> ACTKNAIAQTGFNKDKYFNGDVWYVTDYLDLEPDDVPKRYCAALAAGTASGKLKEALYHYDPKTQDTFYDVSELQVESLGKYTANFKKVDKNGNVKVAVTAGNYYTFTVMYADD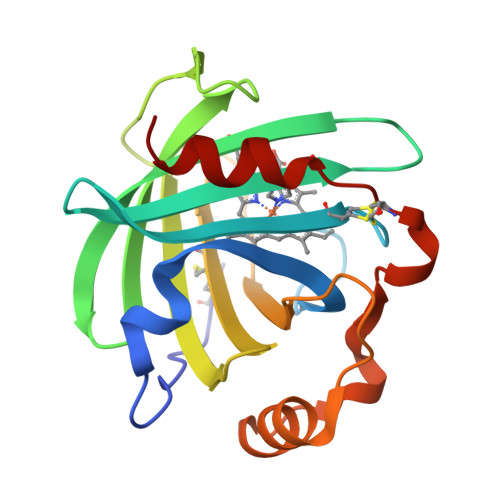SSALIHVCLHKGNKDLGDLYAVLNRNKDAAAGDKVKSAVSAATLEFSKFISTKENNCAYDNDSLKSLLTK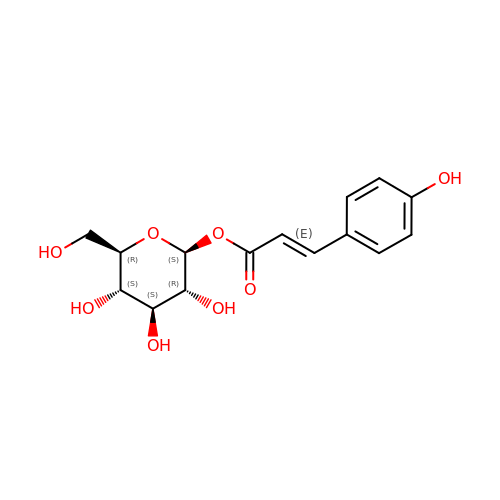p-coumaroyl glucose | C15 H18 O8 | DSNCQKUYZOSARM-QVLXMGEUSA-N> MSYCTLADLIEQYSEQKIREVSDRVNKPATTIDTVIVDRAIADADSEIDLHLHGRYQL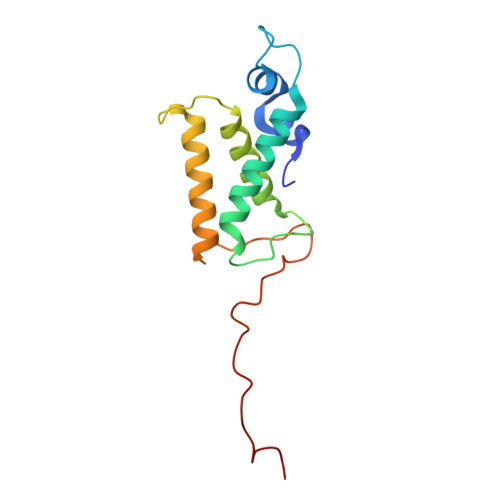PLASVPTALKRIACGLAYANLHIVLKEENPVYKTAEHLRKLLSGIANGKLSLALDADGKPAPVANTVQISEGRNDWGADW A novel enteric T cell superantigen, I2, and its full-length gene product pfiT, are encoded by a microbial gene associated with Crohn's disease (CD). Crystal structure of pfiT at high resolution revealed that pfiT belongs to the bacterial transcription factor family of tetracycline repressor (TetR). We show that pfiT specifically and directly interacts with class II MHC HLA-DR, and to a lesser extent HLA-DP or HLA-DQ, and show that pfiT shares an overlapping binding site on HLA-DR1 with other superantigens. We show that pfiT can stimulate the activation of both mouse splenocytes and human peripheral blood mononuclear cells (PBMCs).

Based upon the high resolution crystal structure of pfiT, we found that pfiT belongs to the TetR transcription regulator protein family. VAST search indicated that pfiT belongs to the TetR-family transcription regulators. TetR proteins function as a dimer to bind their DNA elements. Our results demonstrated that pfiT exists as a dimer in solution; and crystal structure also confirmed that pfiT is a dimer at structural level. Our structural study indicated that the structures of both pfiT and MAM are completely helical, although pfiT displays a different folding pattern. We speculate that the distinct folding patterns might yield differences in molecular contacts that could account for the divergent MHC fine specificities of these two SAgs. The distinct structure of pfiT relative to other SAgs suggests that it represents a novel family of SAg.

> GPLGSMDEHKALGVMRTMVDSGQLTDPESARGKLLQTAAHLFRNKGFERTTVRDLASAVGIQSGSIFHHFKSKDEILRAVMEETIHYNTAMMRASLEEASTVRERVLALIRCELQSIMGGSGEAMAVLVYEWRSLSAEGQAHVLALRDVYEQIWLQVLGEAKAAGYIRGDVFITRRFLTGALSWTTTWFRAQGSLTLEELAEEALLMVLKSD> AVGPVADLTITDAAVSPDGFSRQAVVVNGVTPGPLVAGNIGDRFQLNVIDNLTNHTMLKSTSIHWHGFFQHGTNWADGPAFINQCPISPGHSFLYDFQVPDQAGTFWYHSHLSTQYCDGLRGPFVVYDPNDPHASRYDVDNDDTVITLADWYHTA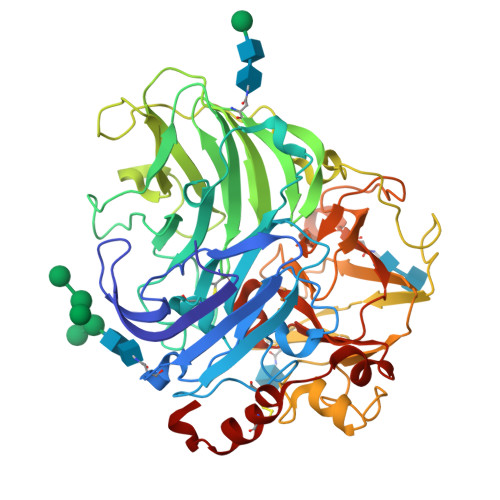AKLGPRFPGGADATLINGKGRAPSDSVAELSVIKVTKGKRYRFRLVSLSCNPNHTFSIDGHNLTIIEVDSVNSQPLEVDSIQIFAAQRYSFVLDANQAVDNYWIRANPNFGNVGFDGGINSAILRYDGAPAVEPTTNQTTSVKPLNEVDLHPLVSTPVPGAPSSGGVDKAINMAFNFNGSNFFINGASFVPPTVPVLLQILSGAQTAQDLLPSGSVYVLPSNASIEISFPATAAAPGAPHPFHLHGHTFAVVRSAGSTVYNYDNPIFRDVVSTGTPAAGDNVTIRFDTNNPGPWFLHCHIDFHLEGGFAVVMAEDTPDVKAVNPVPQAWSDLCPTYDALDPNDQ> GAAAAMSICPHIQQVFQNEKSKDGVLKTCNAARYILNHSVPKEKFLNTMKCGTCHE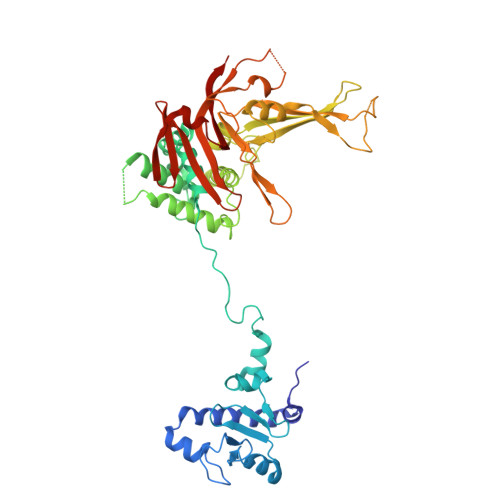INSGATFMCLQCGFCGCWNHSHFLSHSKQIGHIFGINSNNGLLFCFKCEDYIGNIDLINDAILAKYWDDVCTKTMVPSMERRDGLSGLINMGSTCFMSSILQCLIHNPYFIRHSMSQIHSNNCKVRSPDKCFSCALDKIVHELYGALNTKQASSSSTSTNRQTGFIYLLTCAWKINQNLAGYSQQDAHEFWQFIINQIHQSYVLDLPNAKEVSRANNKQCECIVHTVFEGSLESSIVCPGCQNNSKTTIDPFLDLSLDIKDKKKLYECLDSFHKKEQLKDFNYHCGECNSTQDAIKQLGIHKLPSVLVLQLKRFEHLLNGSNRKLDDFIEFPTYLNMKNYCSTKEKDKHSENGKVPDIIYELIGIVSHKGTVNEGHYIAFCKISGGQWFKFNDSMVSSISQEEVLKEQAYLLFYTIRQVN CARBA-GLUCOTROPAEOLIN | C15 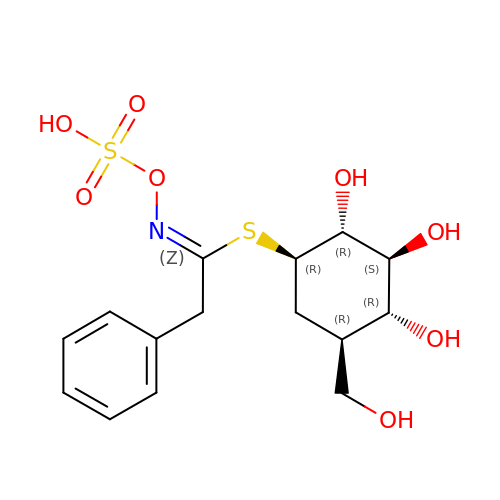H21 N O8 S2 | LZDZCEOFJWRJIA-GGASBGQWSA-N>GKITLYEDRGFQGRHYECSSDHPNLQPYLSRCNSARVDSGCWMLYEQPNYSGLQYFLRRGDYADHQQWMGLSDSVRSCRLIPHSGSHRIRLYEREDYRGQMIEFTEDCSCLQDRFRFNEIHSLNVLEGSWVLY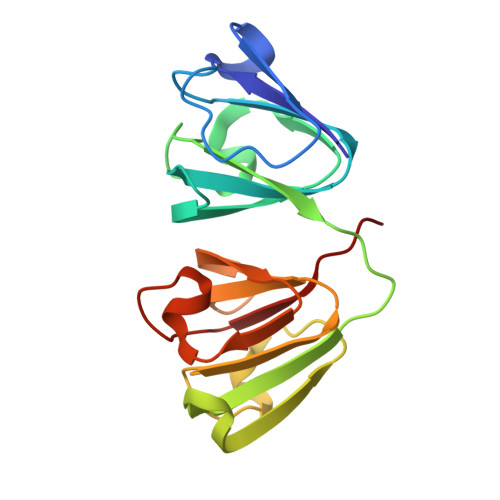ELSNYRGRQYLLMPGDYRRYQDWGATDARVGSLRRVIDFS[2x]>SVSSIVSRAQFDRMLLHRNDGACQAKGFYTYDAFVAAAAAFSGFGTTGSADVQKREVAAFLAQTSHETTGGWATAPDGAFAWGYCFKQERGASSDYCTPSAQWPCAPGKRYYGRGPIQLSHNYNYGPAGRAIGVDLLANPDL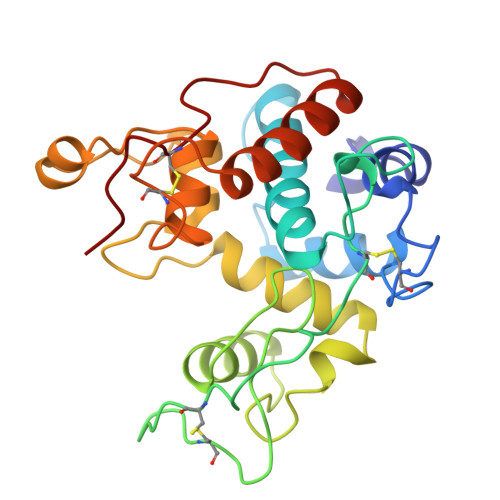VATDATVSFKTAMWFWMTAQPPKPSSHAVIVGQWSPSGADRAAGRVPGFGVITNIINGGIECGHGQDSRVADRIGFYKRYCDILGVGYGNNLDCYSQRPFA[2x]Cytochrome P450 CYP152s catalyze decarboxylation of fatty acids to generate terminal alkenes, valuable compounds for various industries. Here, we identified, overexpressed, and characterized a new CYP152 enzyme from Lacicoccus alkaliphilus (OleTLA) and compared its biophysical and biochemical properties with the well-studied OleTJE from Jeotgalicoccus sp. 8456. The enzyme can bypass the use of redox partners to supply electrons by efficiently using H2O2 as a co-substrate via a peroxide shunt pathway, enabling a convenient in vitro bioconversion process.

The X-ray structure of OleTLA in complex with icosanoic acid revealed a unique flipped heme and a substrate tunnel configuration which are different than those of other CYP152 decarboxylases. Although the overall architecture of OleTLA: C20FA is similar to that of OleTJE: C20FA, we noted distinct differences between the two enzymes. Significant distinctions were observed in the FG-loop region (residue 173–175 of OleTLA) and the β-sheet (residue 388–391 and 413–419 of OleTLA) at the C-terminal. The electron density in these regions, particularly at the FG-loop region, was less defined, indicating greater flexibility in the OleTLA structure compared to OleTJE. OleTLA is notably different from OleTJE and almost all other CYP152s in its heme orientation. The cavity sizes of OleTLA and CYP152N1, which have unusual heme binding, were measured as 2693 Å3 and 2637 Å3, respectively, whereas OleTJE which has normal heme binding showed cavities of 1149 Å3. Three tunnels of OleTLA including the main substrate tunnel pointing towards the FG-loop (residues 173–184) and the loop with residues 61 to 83 while four tunnels of OleTJE including the main substrate tunnel pointing toward other two loops (residues 60–71, and 80–83) were identified. We further analyzed Chain B of OleTLA which binds C20FA in comparison to the C20FA binding in OleTJE. In both structures, almost all residues surrounding C20FA are similar in the two enzymes except V76 (I74 in OleTJE), Y296 (F294 in OleTJE), I178 (L176 in OleTJE), I50 (V48 in OleTJE), and I16 (V16 in OleTJE). Notably, I178 in the FG-loop of OleTLA (equivalent to L176 in OleTJE) exhibits a shorter distance to C16 atom of C20FA than does L176 of OleTJE.

>[2x]MATIKKDKGIDNTAKIAKQGYLYTTNQRERLGVKDGVFETRGLGGKRIIILSGKDGAELFYDNDKVERSGTLPKRVVNTLFGKGAIHTTTGKVHVDRKALFMSLMTEGNLQYLRELTRNHWLMNTQRMENMDQVNVYRESIILLTKVGTRWAGVQAPEKEIENIATDMDIMIDSFKAIGSAFKGYRASKAARRRVEDWLEDQIIQTRKGKIHPPKGTALYEFAHWKDYKGEPMDSRLCGIDLMNTFRPLIAINRFIAFGALAMHENPVAREKIKQDDDYAYMFAQEVRRFYPFVPYLPGKVKEDFQYKGYDFEKDTMLAIDIYGTMHDPDVWENPNEFYPERFKDWDGSPFDLIPQGGGDYYTNHRCAGEWMTIIIMQETMKYFASRITYDVPEQDLTVDLNSLPGYVKSGFIIENVREVVDRDLEHHHHHH> MLEISMEQVSASIGNFTVDLFNKLNETNRDKNIFFSPWSISSALALTYLAAKGSTAREMAEVLHFTEAVRAESSSVARPSRGRPKRRRMDPEHEQAENIHSGFKELLTAFNKPRNNYSLRSANRIYVEKTYALLPTYLQLSKKYYKAEPQKVNFKTAPEQSRKEINTWVEKQTESKIKNLLSSDDVKATTRLILVNAIYFKAEWEVKFQAEKTSIQPFRLSKNKSKPVKMMYMRDTFPVLIMEKMNFKMIELPYVKRELSMFILLPDDIKDGTTGLEQLERELTYERLSEWADSKMMTETLVDLHLPKFSLEDRIDLRDTLRNMGMTTAFTTNADFRGMTDKKDLAISKVIHQSFVAVDEKGTEAAAATAVIISF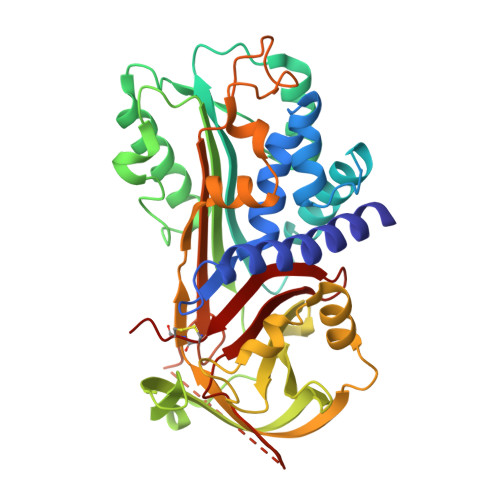TTSVINHVLKFKVDHPFHFFIRHNKSKTILFFGRFCCPVE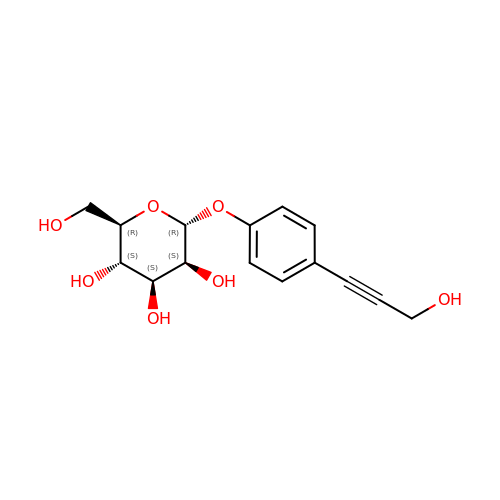4-(3-hydroxyprop-1-yn-1-yl)phenyl alpha-D-mannopyranoside | C15 H18 O7 | GNTPQQUJBAFHOR-MRLBHPIUSA-N DUSP22 is a small phosphatase containing 184 residues, and the sequence contains a catalytic domain as well as an N-terminal myristoylation site. This enzyme is broadly expressed in different tissues and plays important roles in the regulation of signaling pathways, such as inactivating the T cell receptor (TCR) signaling pathway, activating the JNK signaling pathway, and regulating the phosphorylation of focal adhesion kinase (FAK). The phosphatase domain of DUSP22 consists of five twisted β-sheets and six α-helices, and the structural scaffold is similar to that of DUSP3 (VHR), while DUSP22 does not contain an N-terminal α-helix surrounded by the N-loop. In this region, the catalytic activity is facilitated by C88 in the P-loop and D57 in the D-loop, and the hydrogen bonding network is formed by D57 in the D-loop, S93 in the P-loop, and N128 in the N-loop.

The crystal structures of C88S, C88S/S93A, C88S/S93N, WT_VO4, N128A, and N128D were determined in this study. All of the structures contained a ligand, PO4, VO4, or SO4, bound to the P-loop in the active site. The binding of the pTyr-like ligand was representative of the first step in the catalytic reaction, and the binding of vanadate represented the second step. Unlike Q262 in PTP1B, N128 did not rotate to stabilize water during the two catalytic steps. The DPN–triloop interaction was maintained in the catalytic reaction, suggesting that the stable interaction among the three loops was necessary for catalysis. Structural alignment among N128A, N128D, and WT_VO4 revealed that N128 participated in forming the conformation of the D-loop.

> GPMGNGMNKILPGLYIGNFKDARDAEQLSKNKVTHILSVHDSARPMLEGVKYLCIPAADSPSQNLTRHFKESIKFIHECRLRGESCLVHCLAGVSRSVTLVIAYIMTVTDFGWEDALHTVRAGRSCANPNVGFQRQLQEFEKHEVHQYRQWLKEEYG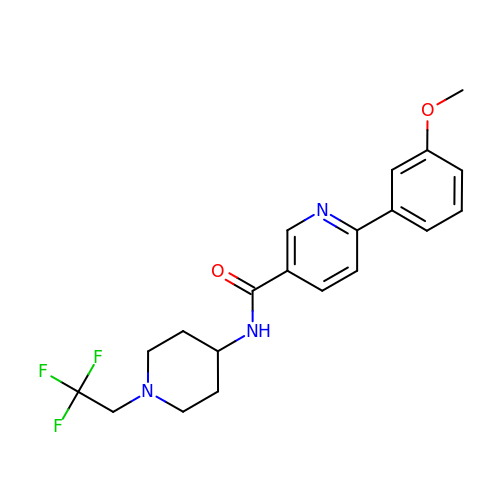6-(3-methoxyphenyl)-N-[1-(2,2,2-trifluoroethyl)piperidin-4-yl]pyridine-3-carboxamide | C20 H22 F3 N3 O2 | KJXMFUFGGQJXRP-UHFFFAOYSA-N>GAASYEKEKELCVKYFEQWSESDQVEFVEHLISQMCH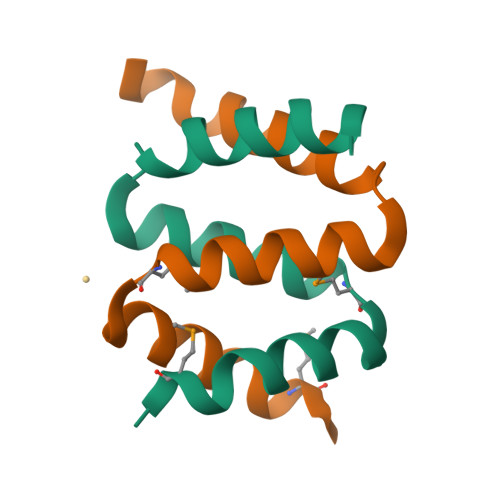YQHGHINSYLKPMLQ[2x]>GPAMNSVFSGLDMLILLPYERRGTRLVVEDYRPDHIYCIGADFGKNQDYSVFSVLDLDTGAIACLERMNGATWSDQVARLKALSEDYGHAYVVADTWGVGDAIAEELDAQGINYTPLPVKSSSVKEQLISN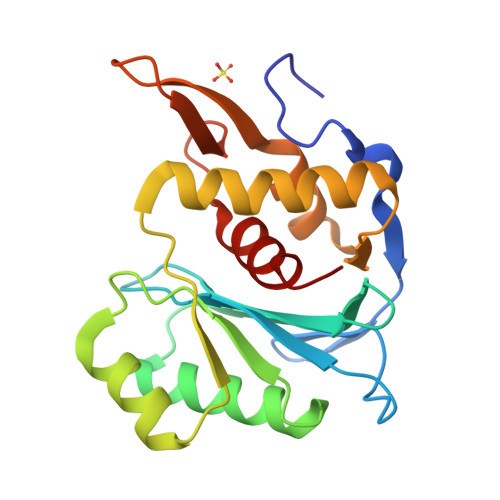LALLMEKGQVAVPNDKTILDELRNFRYYRTASGNQVMRAYGRGHDDIVMSLALAYSQYEG[2x]> MSLNTPFSIDEVSFRDLPGWGQDDPRKLFPAMATILSHLRNAKPYRTGALGITAAELVSLLELAERGQVNSPEQARQFFETNSVPFRISPAQGKSGFVTAFYEPELEVSATPDDVWRYPIYRRPPELVDIDNDNRPDGFDPSYAFGKADEEGISYFPDRRAIDEGCLRGRGLEIAWARSKVDLFFVHVQGAARLVFPDGAIKRITYAAKAGHV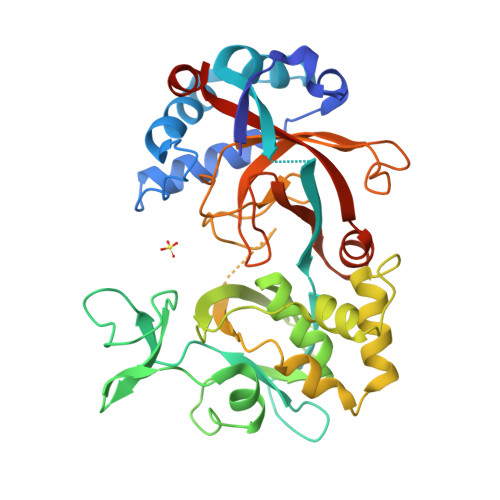FSPIGRLLLDRGELDPKTISMQTIRQWLADHPDEVDGVLWHNRSYIFFREADVAGLDMGPIAAAKVPLVAGRALAVDRLIHTFGLPFFIHAPTLTHLDDGKPFARLMLALDTGSAIVGPARGDIFTGSGFEAGELAGTVRNEADFYILLPRIAAERYRREGHHHHHH> SMEELTLT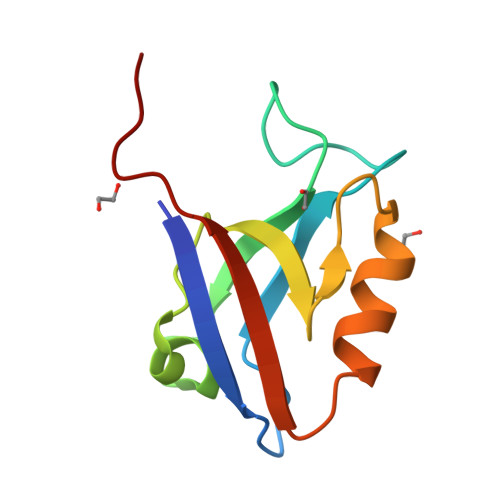ILRQTGGLGISIAGGKGSTPYKGDDEGIFISRVSEEGPAARAGVRVGDKLLEVNGVALQGAEHHEAVEALRGAGTAVQMRVWRERETSV> DRSFRWKYHQFRFLCHSNALPSHVKISVSRQTLFEDSFQQIMNMKPYDLRRRLYIIMRGEEGLDYGGIAREWFFLLSHEVLNPMYCLFEYAGKNNYCLQINPASSINPDHLTYFRFIGRFIAMALYHGKFIDTGFTLPFYKRMLNKRPTLKDLESIDPEFYNSIVWIKENNLEECGLELYFIQDMEILGKVTTHELKEGGESIRVTEENKEEY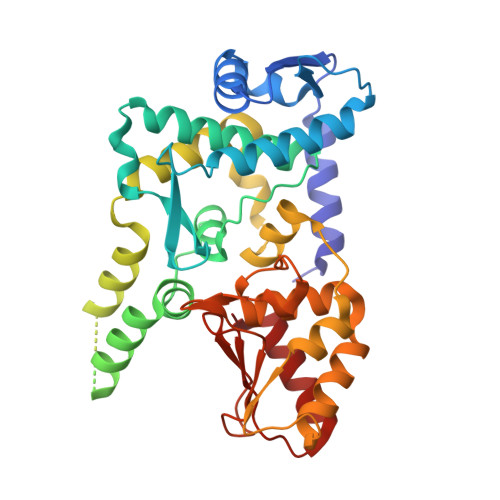IMLLTDWRFTRGVEEQTKAFLDGFNEVAPLEWLRYFDEKELELMLCGMQEIDMSDWQKSTIYRHYTKNSKQIQWFWQVVKEMDNEKRIRLLQFVTGTCRLPVGGFAELIGSNGPQKFCIDKVGKETWLPRSHTCFNRLDLPPYKSYEQLREKLLYAIEETE>[4x]MPLAEGSTFAGFTIVRQLGSGGMGEVYLARHPRLPRQDALKVLRADVSADGEYRARF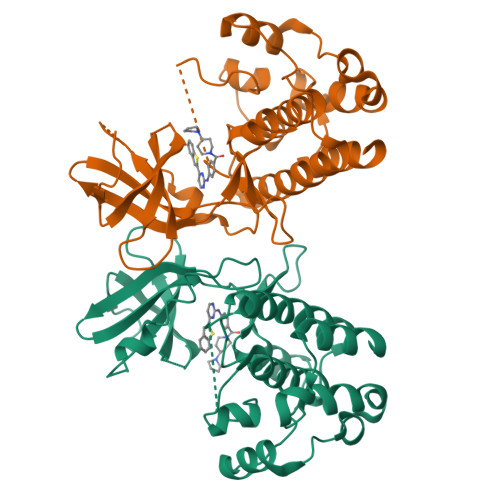NREADAAASLWHPHIVAVHDRGEFDGQLWIDMDFVDGTDTVSLLRDRYPNGMPGPEVTEIITAVAEALDYAHERRLLHRDVKPANILIANPDSPDRRIMLADFGIAGWVDDPSGLTATNMTVGTVSYAAPEQLMGNELDGRADQYALAATAFHLLTGSPPFQHANPAVVISQHLSASPPAIGDRVPELTPLDPVFAKALAKQPKDRYQRCVDFARALGHRL> NPHAKEC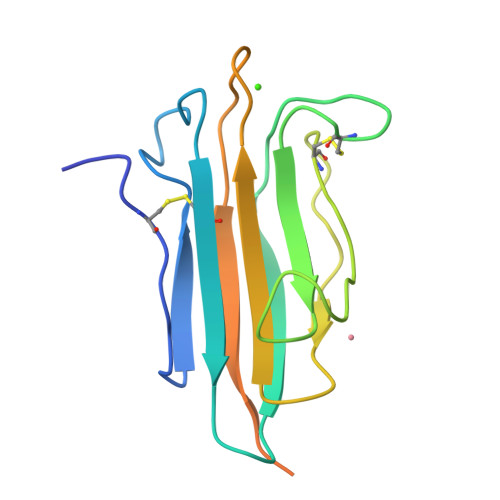GGVFTDPKQIFKSPGFPNEYEDNQICYWHIRLKYGQRIHLSFLDFDLEDDPGCLADYVEIYDSYDDVHGFVGRYCGDELPDDIISTGNVMTLKFLSDASVTAGGFQIKYVAMDPVSKSSQGKNTSTTSTGNKNFLAGRFSHL> GPHMAMGFRLHDLRALLKRICSIQNYTRHVLIEWDVRWVNPLTLASKGWEPYQSASQSQVPFKCCCCHAIMTIPLLKNGDDVADYTMKLNEKIWNSNIIGNHLQKCPW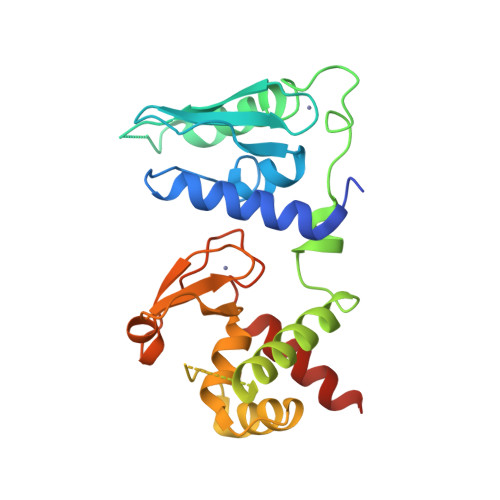RENQVDLNKEYYLSSQNLIREIERIHTEIDRIVSGSNEFSLKRNSSRIFHYLSEKEIQKLAFFFDCKDYSLVGLLLLGYTKFQKDDLVQCTACFHRASLKKLEYTEFNGHALWCRYYNKELLPTMLLELIGKEDKLITK> GSGRMPQSKSRKIAILGYRSVGKSSLTIQFVEGQFVDSYDPTIENTFTKLITVNGQEYHLQLVDTAGQDEYSIFPQTYSIDINGYILVYSVTSIKSFEVIKVIHGKLLDMVGKVQIPIMLVGNKKDLHMERVISYEEGKALAESWNAAFLESSAK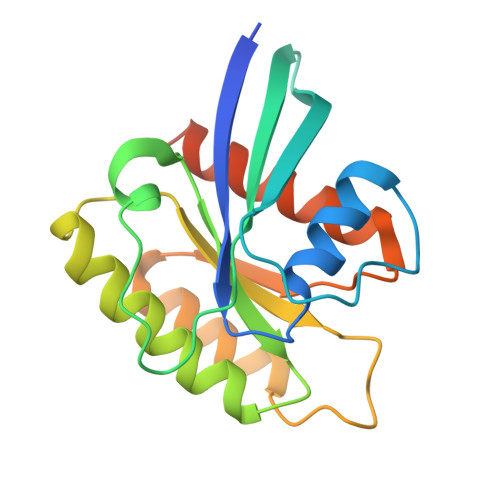ENQTAVDVFRRIILEAEKMDGAASQGKSSCSVM>[4x]GHMKISWNGFSKKSYQERLELLKAQALLSPERQASLEKDEQMSVTVADQLSENVVGTFSL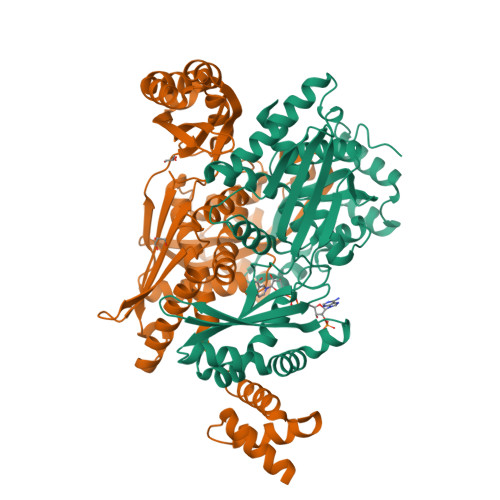PYSLVPEVLVNGQEYTVPYVTEEPSVVAAASYASKIIKRAGGFTAQVHQRQMIGQVALYQVANPKLAQEKIASKKAELLELANQAYPSIVKRGGGARDLHVEQIKGEPDFLVVYIHVDTQEAMGANMLNTMLEALKPVLEELSQGQSLMGILSNYATDSLVTASCRIAFRYLSRQKDQGREIAEKIALASQFAQADPYRAATHNKGIFNGIDAILIATGNDWRAIEAGAHAFASRDGRYQGLSCWTLDLEREELVGEMTLPMPVATKGGSIGLNPRVALSHDLLGNPSARELAQIIESIGLAQNFAALKALVSTGIQQGHMKLQAKSLALLAGASESEVAPLVERLISDKTFNLETAQRYLENLRS>MTDTHTGPTPADAVPAYPFSLPHALDLDPHYAELRRDEPVSRVRLPYGEGTAWLVTRMSDARIVLGDSRFSTAAATDPATPRMFPTPPEPDGVLAQDPPDHTRLRRLVGKAFTARRVEEMRPRVRSLVDSLLDDMVAHGSPADLVEFLAVPFPVAVICELLGVPLEDRDLFRTFSDAMLSSTRLTAAEIQRVQQDFMVYMDGLVAQRRDAPTEDLLGALALATDNDDHLTKGEIVNMGVSLLIAGHETSVNQITNLVHLLLTERKRYESLVADPALVPAAVEEMLRYTPLVSAGSFVRVATEDVELSTVTVRAGEPCVVHFASANRDEEVFDHADELDFHRERNPHIAFGHGAHHCIGAQLGRLELQEALSALVRRFPTLDLAEPVAGLKWKQGMLIRGLERQIVSW[6x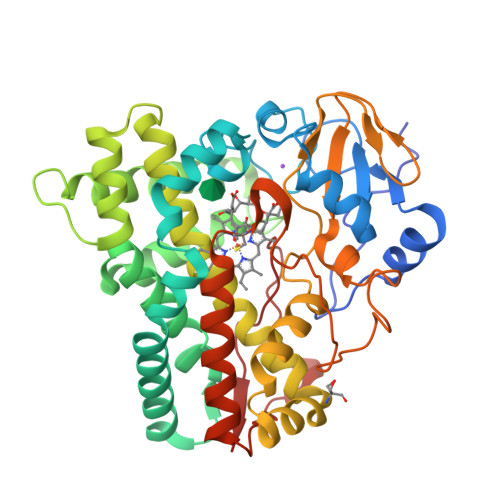]>[6x]M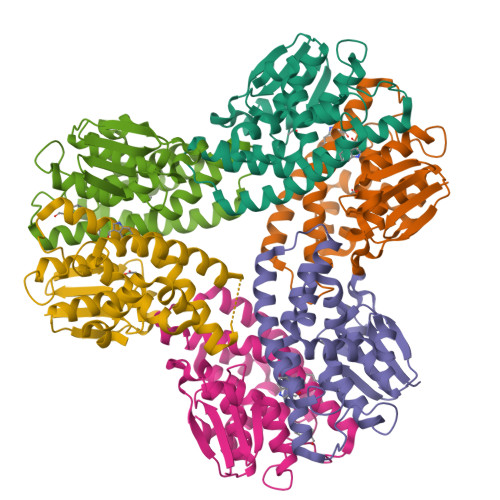AGIKVFGHPASIATRRVLIALHEKNLDFELVHVELKDGEHKKEPFLSRNPFGQVPAFEDGDLKLFESRAITQYIAHRYENQGTNLLQTDSKNISQYAIMAIGMQVEDHQFDPVASKLAFEQIFKSIYGLTTDEAVVAEEEAKLAKVLDVYEARLKEFKYLAGETFTLTDLHHIPAIQYLLGTPTKKLFTERPRVNEWVAEITKRPASEKVQ Transfer RNA–guanine transglycosylase (Tgt, EC 2.4.2.29) catalyses the exchange of a specific guanine base in tRNA molecules by a substituted 7-deazaguanine. Bacterial Tgt functions as a homodimer in which the protomer consists of a (βα)8 barrel harbouring a Zn2+ binding subdomain close to the C-terminus. The reaction follows a ping-pong mechanism including a covalent Tgt⋅tRNA intermediate. Hence, in an attempt to generate a model system for the active site of human Tgt and to gain insights into the relevance of particular amino acids for substrate base selectivity, we adapted the Z. mobilis Tgt active site by site-directed mutagenesis in order to mimic that of the human enzyme.

In order to investigate the importance of Gly232 and Val161 in human Tgt for queuine recognition, we created a doubly mutated variant of the Z. mobilis enzyme in which the corresponding Val233 and Cys158 were exchanged by glycine and valine, respectively. To allow the interpretation of the obtained data at a structural level, we determined the crystal structures of the mutated Tgt variants created in this study in their apo-forms as well as in complex with preQ1 and queuine. The crystal structures of Tgt(Cys158Val) and Tgt(Cys158Val/Val233Gly), each in complex with preQ1, reveal, compared to the corresponding apo-forms, a shift of Val158 towards the ligand. In contrast, this side chain is excellently defined in the electron density maps of apo- and preQ1-bound Tgt(Cys158Val) and Tgt(Cys158Val/Val233Gly).

> MVEATAQETDRPRFSFSIAAREGKARTGTIEMKRGVIRTPAFMPVGTAATVKALKPETVRATGADIILGNTYHLMLRPGAERIAKLGGLHSFMGWDRPILTDSGGFQVMSLSSLTKQSEEGVTFKSHLDGSRHMLSPERSIEIQHLLGSDIVMAFDEVTPYPATPSRAASSMERSMRWAKRSRDAFDSRKEQAENAALFGIQQGSVFENLRQQSADALAEIGFDGYAVGGLAGGEGQDEMFRVLDFSVPMLPDDKPHYLMGVGKPDDIVGAVERGIDMFDCVLPTRSGRNGQAFTWDGPINIRNARFSEDLKPLDSECHCAVCQKWSRAYIHHLIRAGEILGAMLMTEHNIAFYQQLMQKIRDSISEGRFSQFAQDFRARYFARNS>[2x]FQGMEVHVCSVGTSLLKNSLDDDNVRKEIERLGLKDWDRLKFDDDRQNRIKENFDSLRKMLLKFIRSKGRRASAELDSLFSTFEKLKHNKSEIYVFLYSTNTSNSQLAGEVIRDYLIEEGIRSELVTVKTISSEENFYEGIVDLFDKVIYRILKFKEQDNEVYINATPGLKP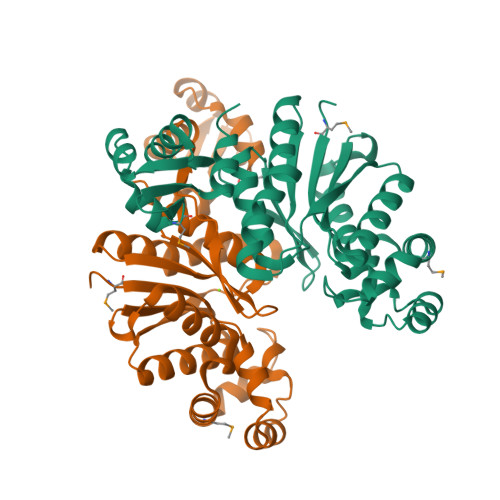ESIFLTLAGLLAGADLIYYKYQEFNDVVILPSPPITIRPKYLDWLIRFAISGYTLSEKRAEELGIPVRLLEAKMLVERKGEDAYRLKDWVRKLLGIYLPIGAQNKYYRVIVEGEGERTFDNEVEAYNYMESKRKEGKNVRVEVPDRVYFLGL> GSLFQLKRETDDLEQWISEKELVASSPEMGQDFDHVTLLRDKFRDFARETGAIGQERVDNVNAFIERLIDAGHSEAATIAEWKDGLNEMWADLLELIDTRMQLLAASYDLHRYFYTGAEILGLIDEKHRELPEDVGLDASTAESFHRVHTAFERELHLLGVQVQQFQDVATRLQT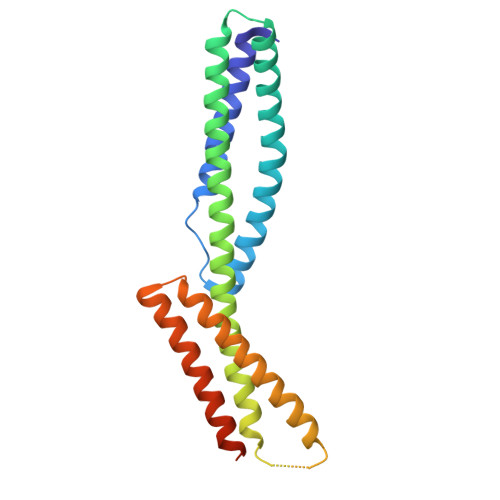AYAGEKAEAIQNKEQEVSAAWQALLDACAGRRTQLVDTADKFR> GPGGEMQKIVFKIPMVDDKSRTKAMSLVAST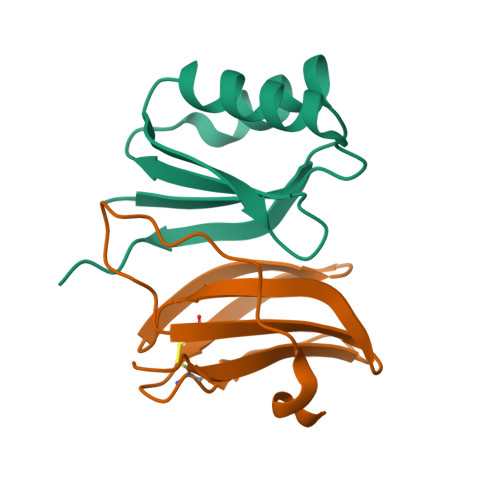VGVHSVAIAGDLRDQVVVVGDGIDSINLVSALRKKVGPAMFLEVSQVKED;> METGNKYIEKRAIDLSRERDPNFFDNADIPVPECFWFMFKNNVRQDAGTCYSSWKMDMKVGPNWVHIKSDDNCNLSGDFPPGWIVLGKKRPGF>MSKLASPQSVRALLERHGLFADKRFGQNFLVSEAHLRRIVEAARPFTGPVFEVGPGLGALTRALLEAGAEVTAIEKDLRLRPVLEETLSGLPVRLVFQDALLYPWEEVPQGSLLVANLPYHIATPLVTRLLKTGRFARLVFLVQKEVAERMTARPKTPAYGVLTLRVAHHAVAERLFDLPPGAFFPPPKVWSSLVRLTPTGALDDPGLFRLVEAAFGKRRKTLLNALAAAGYPKARV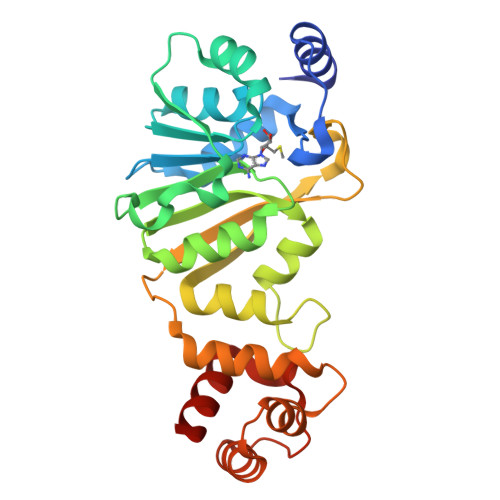EEALRALGLPPRVRAEELDLEAFRRLREGLEGAV[3x]N,N,N-trimethyl-2-phosphonoethan-1-aminium 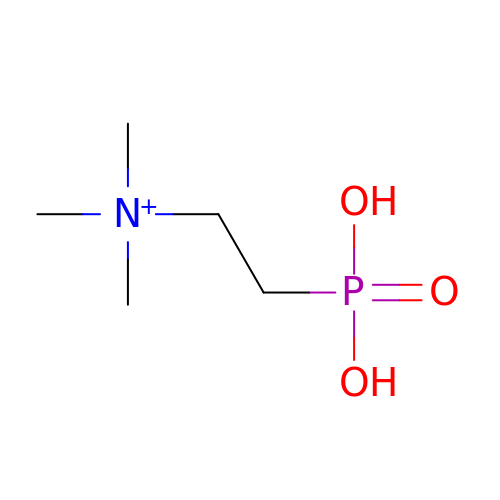| C5 H15 N O3 P | VCANKBLUHKRQLL-UHFFFAOYSA-O> GPLGSEAAPEYRVIVDANNLTVEIENELNIIHKFIRDKYSKRFPELESLVPNALDYIRTVKELGNSLDKCKNNENLQQILTNATIMVVSVTASTTQGQQLSEEELERLEEACDMALELNASKHRIYEYVESRMSFIAPNLSIIIGASTAAKIMG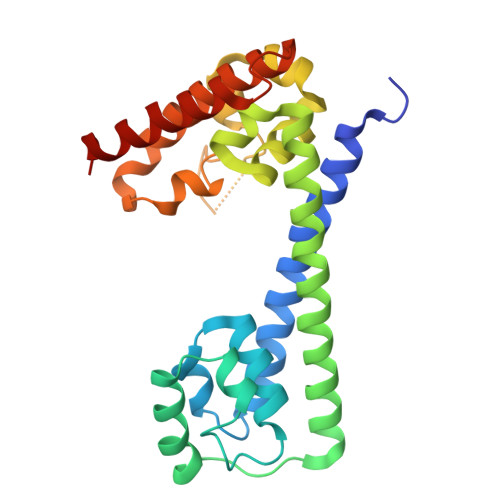VAGGLTNLSKMPACNIMLLGAQRKTLSGFSSTSVLPHTGYIYHSDIVQSLPPDLRRKAARLVAAKCTLAARVDSFHESTEGKVGYELKDEIERKFDKWQE> MNYTKFDVKNWVRREHFEFYRHRLPCG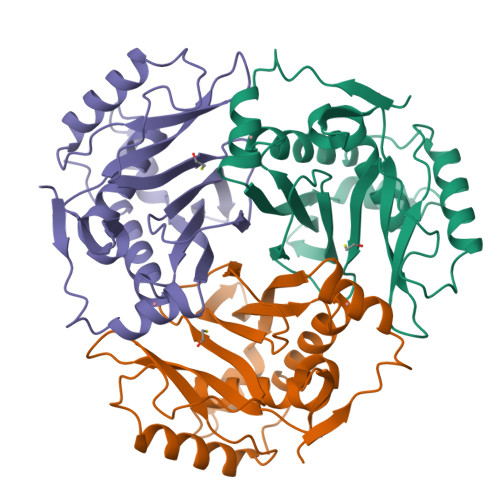FSLTSKIDITTLKKSLDDSAYKFYPVMIYLIAQAVNQFDELRMAIKDDELIVWDSVDPQFTVFHQETETFSALSCPYSSDIDQFMVNYLSVMERYKSDTKLFPQGVTPENHLNISALPWVNFDSFNLNVANFTDYFAPIITMAKYQQEGDRLLLPLSVQVHQAVCDGFHVARFINRLQELCNSKLK To import molecules that are too large for diffusion through outer-membrane porins, bacteria employ a diverse family of membrane proteins termed TonB-dependent transporters (TBDTs; Noinaj et al., 2010). These transporters in the outer membrane are so named because they engage in active transport, the energy for which is provided by the TonB–ExbBD complex in the inner membrane, which spans the periplasm to interact with TBDTs. The final TBDT possessed by E. coli K12 is YncD, and the substrate of this transporter remains unknown. The homolog of YncD in Salmonella enterica ssp. enterica serovar Typhi (Salmonella Typhi) has been shown to be important for virulence in a mouse model of infection.

To gain insight into the evolutionary relationship between YncD and other TBDTs and to provide clues to the nature of the YncD substrate, we solved the crystal structure of YncD by X-ray crystallography. The diffraction from YncD crystals exhibited significant anisotropy. Diffraction data were processed and scaled anisotropically using the diffraction anisotropy server with a final maximum resolution of between 2.96 and 3.5 Å, depending on the reciprocal-lattice direction. However, this solution did not provide sufficient phasing power for model improvement. To obtain experimental phases, YncD crystals were soaked with potassium tetranitroplatinate and anomalous diffraction data were collected to 3.5 Å resolution. Phases were obtained for this data set using single-wavelength anomalous dispersion phasing in combination with molecular replacement using the FecA-derived model (MR-SAD). An initial model of YncD was built using maps from this data set and was utilized to obtain phases for the higher resolution data set by molecular replacement. The structure of YncD was then built and refined using the anisotropically truncated native data. The DALI server was utilized to search the PDB for structural homologues of YncD, revealing that the closest structural homologue to YncD is FecA, which is consistent with our sequence analysis. Despite the low sequence identity of 21% between YncD and FecA, these proteins share a backbone-atom root-mean-square deviation (r.m.s.d.) of 2.2 Å. We determined the crystal structure of YncD, demonstrating that it possesses a compact positively charged extracellular substrate-binding site that is characteristic of TBDTs that import negatively charged small-molecule substrates. Based on its compact positively charged extracellular binding site, the substrate of YncD is likely to be relatively small and negatively charged.

> MKIFSVRQTVLPALLVLSPVVFAADEQTMIVSAAPQVVSELDTPAAVSVVDGEEMRLATPRINLSESLTGVPGLQVQNRQNYAQDLQLSIRGFGSRSTYGIRGIRLYVDGIPATMPDGQGQTSNIDLSSVQNVEVLRGPFSALYGNASGGVMNVTTQTGQQPPTIEASSYYGSFGSWRYGLKATGATGDGTQPGDVDYTVSTTRFTTHGYRDHSGAQKNLANAKLGVRIDEASKLSLIFNSVDIKADDPGGLTKAEWKANPQQAPRAEQYDTRKTIKQTQAGLRYERSLSSRDDMSVMMYAGERETTQYQSIPMAPQLNPSHAGGVITLQRHYQGIDSRWTHRGELGVPVTFTTGLNYENMSENRKGYNNFRLNSGMPEYGQKGELRRDERNLMWNIDPYLQTQWQLSEKLSLDAGVRYSSVWFDSNDHYVTPGNGDDSGDASYHKWLPAGSLKYAMTDAWNIYLAAGRGFETPTINELSYRADGQSGMNLGLKPSTNDTIEIGSKTRIGDGLLSLALFQTDTDDEIVVDSSSGGRTTYKNAGKTRRQGAELAWDQRFAGDFRVNASWTWLDATYRSNVCNEQDCNGNRMPGIARNMGFASIGYVPEDGWYAGTEARYMGDIMADDENTAKAPSYTLVGLFTGYKYNYHNLTVDLFGRVDNLFDKEYVGSVIVNESNGRYYEPSPGRNYGVGMNIAWRFE> GPGEQESDIDEFDLLEGDEKLPGDSELDKTTSIYPPETSWEVNKGMNSSRLHKLYSLFFDKSSAFYLGDDVSVLEDKPLTGAYGFQSKKNDQQIFLFRPDSDYVAGYHVDAKSDAGWVNDKLDRRLSEISEFCSKATQPATFILPFVEMPTDITKGVQHQVLLTISYDPKSKQLTPTVYDSIGRDTYSESLSSYFKGKYRTTCDEILTQSIEKAIKSTDFTLGKFTRAAYNHQNRLTEGNCGSYTFRTIKEVISSSAQGTEVKIPGSGYITSNSYLTSQHVQDIESCIKYRNLGVVDIESALTEGKTLPVQLSEFIVALEDYGKLRSQQSEKSMLNFIGYSKTAKLTAVELLIGILNDIKGKNEISESQYDKLVKEVDCLMDSSLGKLVQFHLKNLGAESLQKLVLPCVKFDDTIDDFVTIE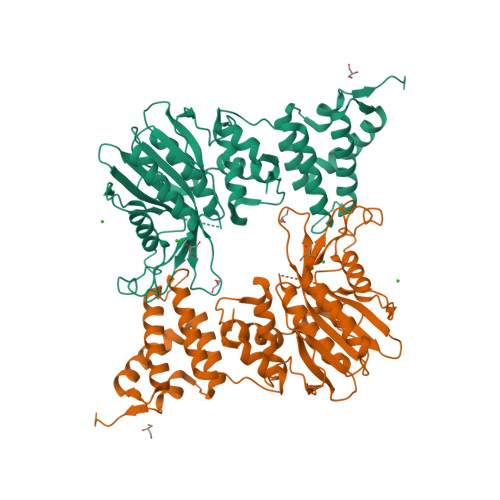KDELFDVPDITGEELASKKGIEQGALDKEALLKQKQIKTDLLDLREEDKTGLKKPLHGGIKVK>[2x]MVENSELRKAGLKVTLPR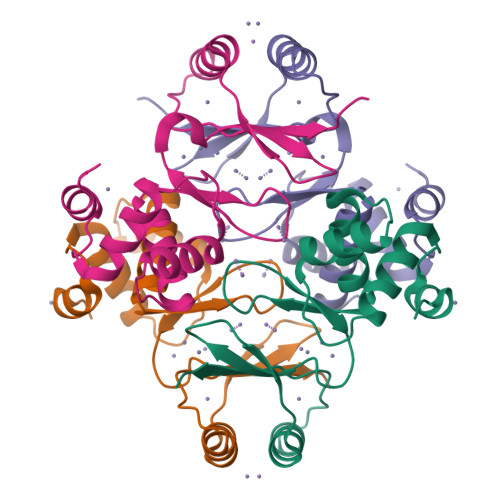VKILQMLDSAEQRHMSAEDVYKALMEAGEDVGLATVYRVLTQFEAAGLVVRHNFDGGHAVFELADSGAHDHMVCVDTGEVIEFMDAEIEKRQKEIVRERGFELVDANLVLYVRKKK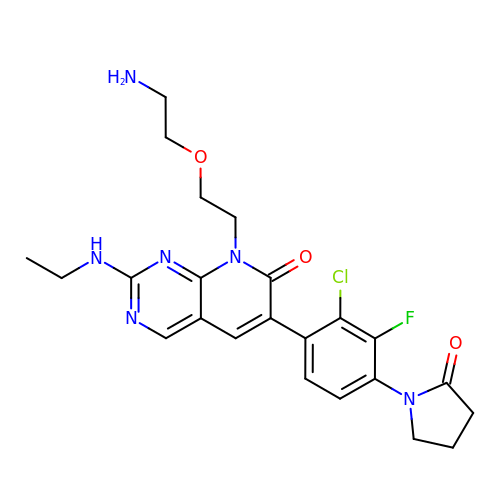(6M)-8-[2-(2-aminoethoxy)ethyl]-6-[2-chloro-3-fluoro-4-(2-oxopyrrolidin-1-yl)phenyl]-2-(ethylamino)pyrido[2,3-d]pyrimidin-7(8H)-one | C23 H26 Cl F N6 O3 | KFVPRGMMTHBEBX-UHFFFAOYSA-N> MNRAFSRKKDKTWMHTPEALSKHFIPYNAKFLGSTEVEQPKGTEVVRDAVRKLKFARHIKKSEGQKIPKVELQISIYGVKILEPKTKEVQHNCQLHRISFCADDKTDKRIFTFICK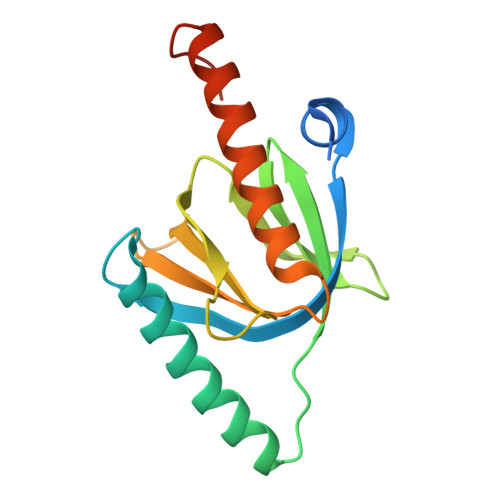DSESNKHLCYVFDSEKCAEEITLTIGQAFDLAYRKFLESGGKDVETRKQIAG>[12x]MSTPGAQEVLFRTGIAAVNSTNHLRVYFQDSHGSIRESLYESGWANGTAKNVIAKAKLGTPLAATSKELKNIRVYSLTEDNVLQEAAYDSGSGWYNGALAGAKFTVAPYSRIGSVFLAGTNALQLRIYAQKTDNTIQEYMWNGDGWKEGTNLG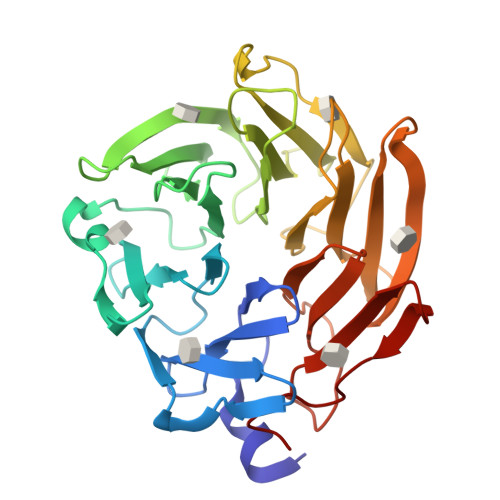VALPGTGIGVTCWRYTDYDGPSIRVWFQTDNLKLVQRAYDPHTGWYKELTTIFDKAPPRCAIAATNFNPGKSSIYMRIYFVNSDNTIWQVCWDHGQGYHDKRTITPVIQGSEIAIISWEGPELRLYFQNGTYVSAISEWTWGKAHGSQLGRRALPPAE>SHGMAVTKVTVDGIEFPPTITPPGSSKSLTLLGAGVRGMEIETIQIKVTAIGVYAEPEVIASHLQKWKGKSASELVEDDGFFKDLVQAPVEKLVKITIIKGIKGSQYGGAVEESIRDRLAALDKYSEAEEEALEEFREFFQTKSLPKGSVIFFHWPSPSTLQISVSTDG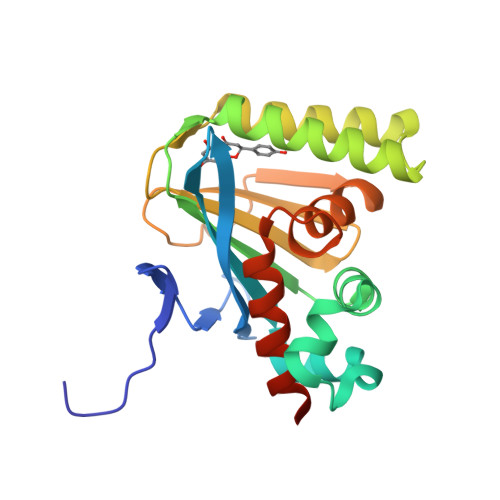SLPEEAEATVENANVAAALLDVFLGENSVSPSTKASVAEGISALLMKNKDEKEV[2x]>[4x]MA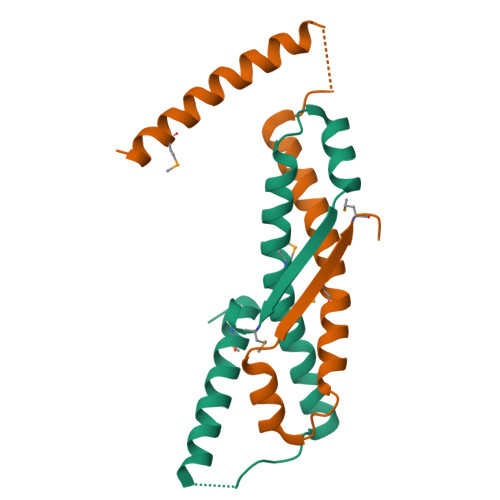SKKPDKTYEEMVKEVERLKLENKTLKQKVKSSGAVSSDDSILTAAKRESIIVSSSRALGAVAMRKIEAKVRSRAAKAVTEQELTSLLQSLTLRVDVSMEELEHHHHHH>GSHMVPDTPTRLVFSALG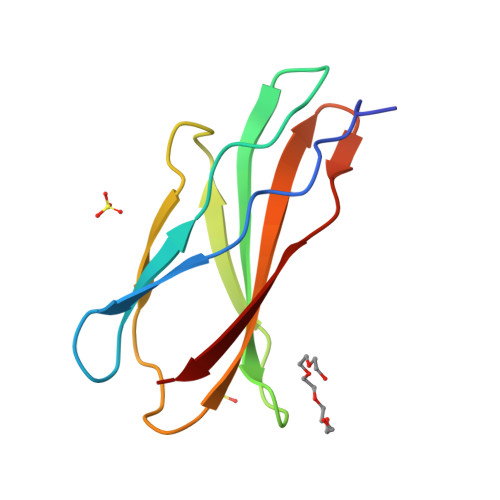PTSLRVSWQEPRCERPLQGYSVEYQLLNGGELHRLNIPNPAQTSVVVEDLLPNHSYVFRVRAQSQEGWGREREGVITI[2x]>GMDLHSLLELGTKPTAPHVRNKKVILFDTNHQVSICNQIIDAINSGIDLGDLLEGGLLTLCVEHYYNSDKDKFNTSPIAKYLRDAGYEFDVIKNADATRFLDVIPNEPHYSPLILALKTLESTESQRGRIGLFLSFCSLFLPKLVVGDRASIEKALRQVTVHQEQGIVTYPNHWLTTGHMKVIFGILRSSFILKFVLIHQGVNLVTGHDAYDSIISNSVGQTRFSGLLIVKTVLE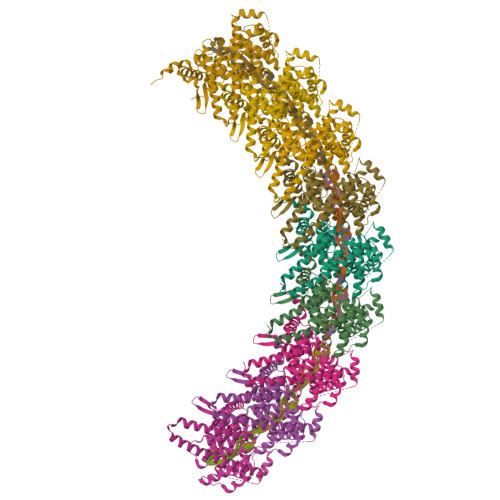FILQKTDSGVTLHPLVRTSKVKNEVASFKQALSNLARHGEYAPFARVLNLSGINNLEHGLYPQLSAIALGVATAHGSTLAGVNVGEQYQQLREAAHDAEVKLQRRHEHQEIQAIAEDDEERKILEQFHLQKTEITHSQTLAVLSQKREKLARLAAEIENNIVEDQGFKQSQNRVSQSFLNDPTPVEVTVQARPMNRVEHHHHHHHH[3x]>MCATKSDNTLIFNISLDHNADTSIEKFFTVFSKKLSGKLNKKINVNFNIVDDSFTKINNIQANKADFAFVNSQAIASNNWFGYTPLIQTLTTAFKEDLELDYYEDGNLQKKAEKTNLLFLSPPYKEWDDIKQKWTGNRYDFLYEPSKLVSFYRSMILITGSASEITAIKKAWNEKNWNQFMKFGIGHGQTNSASRFELPDLLFRKHFAKNYPGLQNAINSDPDKFAVVRGREIGINKNIKIVFDDANSFSWTQNIKGSKRPFYTPIDPNDRLEILTYSDPLLYDIGIVSNNLSRIYQKAIGEIFIELAQSSEDLYGPSIGYNGYKMINDFEKEVVEIIEKTYG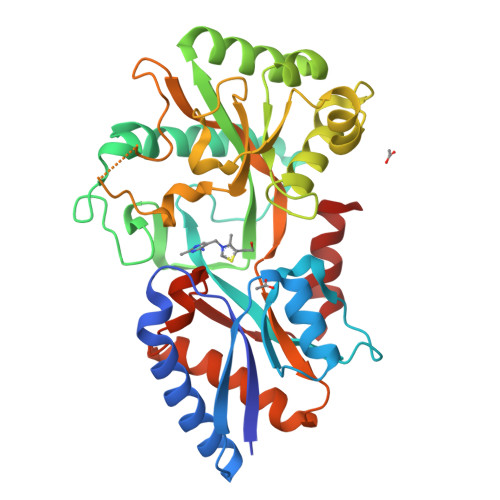K[2x]> HSNEKWFHGKLGAGRDGRHIAERLLTEYCIETGAPDGSFLVRESETFVGDYTLSFWRNGKVQHCRIHSRQDAGTPK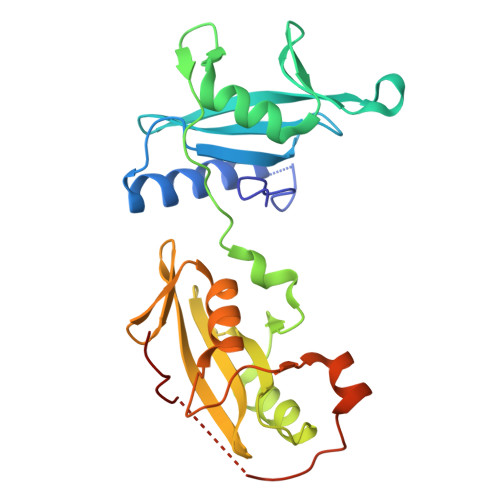FFLTDNLVFDSLYDLITHYQQVPLRCNEFEMRLSEPVPQTNAHESKEWYHASLTRAQAEHMLMRVPRDGAFLVRKRNEPNSYAISFRAEGKIKHCRVQQEGQTVMLGNSEFDSLVDLISYYEKHPLYRKMKLRYPINEEALEKIGTAEPDYGALYEGRNPGFYVEANPMP>GSHMSPSERQCVETVVNMGYSYECVLRAMKAAGANIEQILDYLFAHGQLCEKGFDPLLVEEALEMHQCSEEKMMEFLQLMSKFKEMGFELKDIKEVLLLHNNDQDNALEDLMARAGAS[2x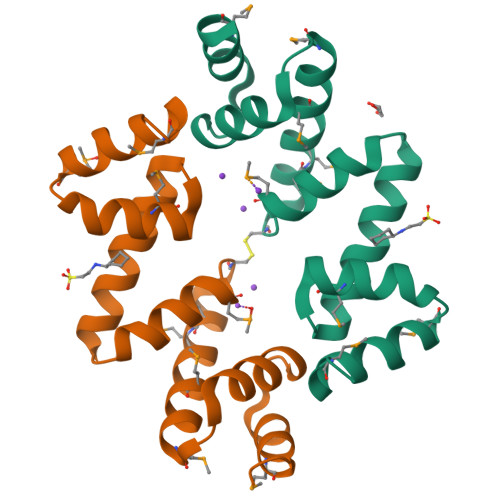]(3aR,5R,6S,7R,7aR)-2-amino-5-(hydroxymethyl)-5,6,7,7a-tetrahydro-3aH-pyrano[3,2-d][1,3]thiazole-6,7-diol 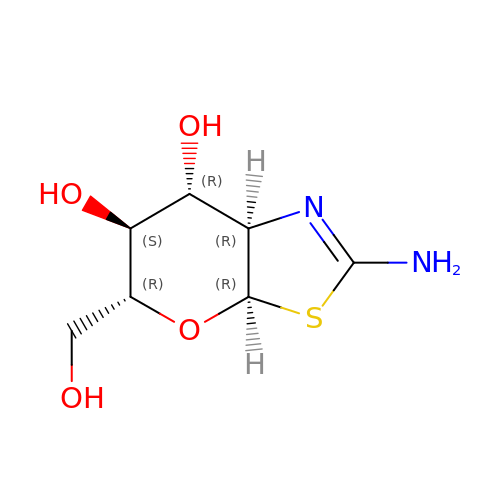| C7 H12 N2 O4 S | PUFNZEXJKQHIQN-QZABAPFNSA-N> AAPKAPADGLKMDKTKQPVVFNHSTHKAVKCGDCHHPVNGKKDYQKCATAGCHDNMDKKDKSAKGYYHAMHDKGTKFKSCVGCHLETAGADAAKKKELT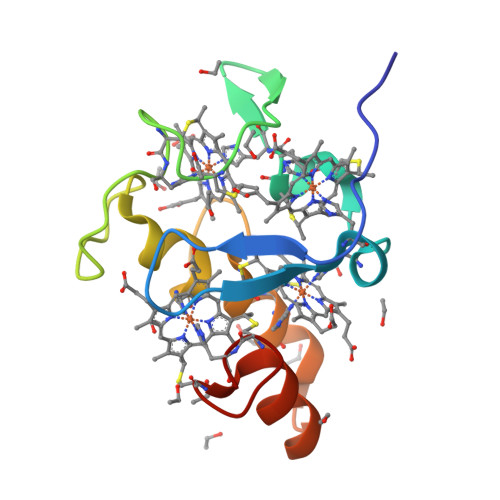GCKGSKCHS> MILSDKDIIDYVTSKRIIIKPFNKDFVGPCSYDVTLGDEFIIYDDEVYDLSKELNYKRIKI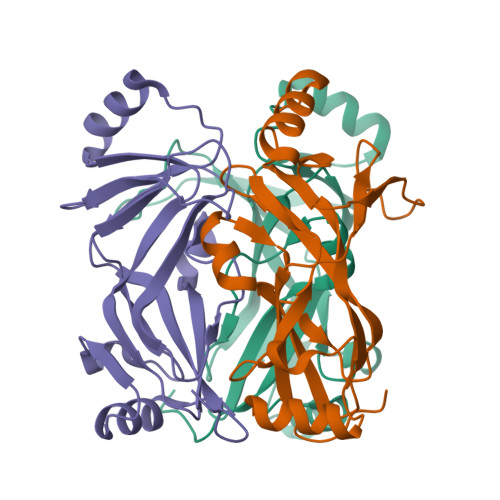KNSILVCPLNYNLTEEKINYFKEKYNVDYVVEGGVLGTTNEYIELPNDISAQYQGRSSLGRVFLTSHQTAGWIDAGFKGKITLEIVAFDKPVILYKNQRIGQLIFSKLLSPADVGYSERKTSKYAYQKSVMPSLIHLDNHKKD>MGKAVIAIHGGAGAISRAQMSLQQELRYIEALSAIVETGQKMLEAGESALDVVTEAVRLLEECPLFNAGIGAVFTRDETHELDACVMDGNTLKAGAVAGVSHLRNPVLAARLVMEQSPHVMMIGEGAENFAFARGMERVSPEIFSTSLRYEQLLAARKEGATVLDHSGAPLDEKQKMG[2x];>[2x]TVGAVALDLDGNLAAATSTGGMTNKLPSTVGSSPLVGAGCYANNASVAVSCTGTGEVFIRALAAYDIAALMDYGGLSLAEACERVVMEKLPALGGSGGLIAIDHEG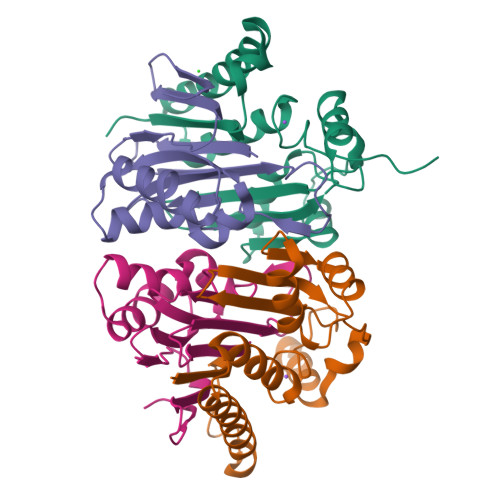NVALPFNTEGMYRAWGYAGDTPTTGIYREKGDTVATQ PLK4, and this interaction targets STIL to centrioles. allows homo-multimerisation, the interaction with the PB3 domain of PLK4, or both. structures and interactions of CCDs and PLK4-PB3s in humans and flies. STIL/Ana2, which can then interact with and recruit Sas-6.

1.53 Å shown in green in cartoon representation. six-stranded beta sheet with an alpha helix packed against one side. behaved as a monomer in solution. Drosophila PB3 and CCD do not detectably interact. equivalent fly proteins do not interact in this way. results suggest that its function may differ between species. humans but is regulated in flies, perhaps by post-translational regulation.

>GPMGQNIPIKRINVPEIGIATELSHGVVQVQFYDGSVVSVIPSMQGGGITYTQPNGTSTHFGKGDDLPFPVRDRVGQIPNIQLKLKTAPLLGS[2x]> MESLTLQPIARVDGTINLPGSKTVSNRALLLAALAHGKTVLTNLLDSDDVRHMLNALTALGVSYTLSADRTRCEIIGNGGPLHAEGALELFLGNAGTAMRPLAAALCLGSNDIVLTGEPRMKERPIGHLVDALRLGGAKITYLEQENYPPLRLQGGFTGGNVDVDGSVSSQFLTALLMTAPLAPEDTV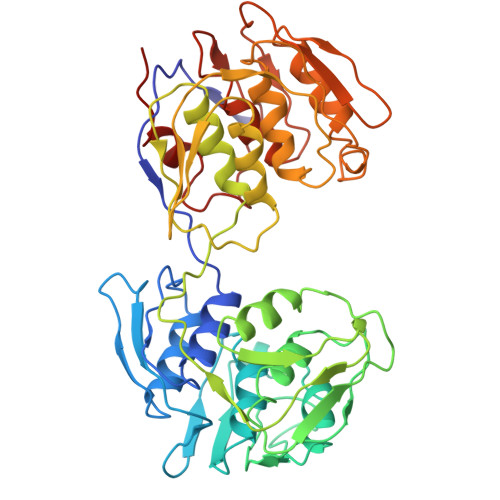IRIKGDLVSKPYIDITLNLMKTFGVEIENQHYQQFVVKGGQSYQSPGTYLVEGDASSASYFLAAAAIKGGTVKVTGIGRNSMQGDIRFADVLEKMGATICWGDDYISCTRGELNAIDMDMNHIPDAAMTIATAALFAKGTTRLRNIYNWRVKETDRLFAMATELRKVGAEVEEGHDYIRITPPEKLNFAEIATYNDHRMAMCFSLVALSDTPVTILDPKCTAKTFPDYFEQLARISQAA> MKKISLLLICLLITTFAKAQDIERPITTGVP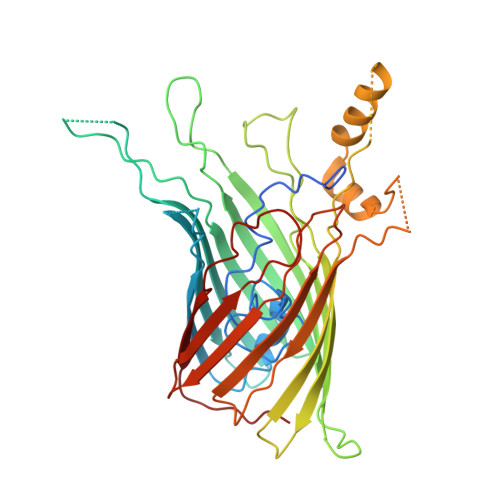FLLVAADARAAGLGDQGVATSSDVFSQQWNPAKYAFAEDAQGLSISYTPYLTDLANDISLGQVTYYNKINDRSAFAGSFRYFGFGGIELRQTGDPNEPTREVNPNEFALDGSYSLKLSETFSMAVAARYIRSNLKVATEEIDASAAGSFAVDVAGFYQSEEIAYSDFNGRWRAGFNIQNLGPKISYDHDDLSANFLPANLRVGGGFDFIFDDYNKLGVSLELTKLLVPTPPGPGTPYDANGDGDFTDPGDISQSQADEANYKKYKDIGWVSGIFKSFGDAPGGFSEELKEITYSAAAEYMYQDAFAMRLGYYHESPMKGAKQFFSLGAGFKYSMIKVDVSYLFSASKVKNPLENTLRFSLTFNFGDKYETY> MEHVAFGSEDIENTLAKMDDGQLDGLAXGAIQLDGDGNILQYNAAEGDITGRDPKQVIGKNFFKDVAPCTDSPEFYGKFKEGVASGNLNTMFE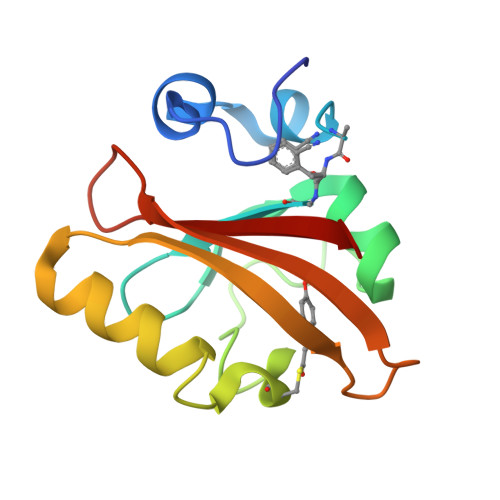YTFDYQMTPTKVKVHMKKALSGDSYWVFVKRV Retinoid-related orphan receptor gamma (RORγ) is a transcription factor belonging to a sub-family of nuclear receptors that includes two closely related members RORα and RORβ. The nuclear hormone receptor RORγ regulates transcriptional genes involved in the production of the pro-inflammatory interleukin IL-17 which has been linked to autoimmune diseases such as rheumatoid arthritis, multiple sclerosis and inflammatory bowel disease. This transcriptional activity of RORγ is modulated through a protein-protein interaction involving the activation function 2 (AF2) helix on the ligand binding domain of RORγ and a conserved LXXLL helix motif on coactivator proteins. The conformation of the AF2 helix can be modulated through targeted ligands which bind the LBS and increase the binding of the coactivator protein (agonists) or disrupt binding (inverse agonists) thereby enhancing or inhibiting transcription.

However, extensive crystallization efforts with BIO399 and RORγ518 or other AF2 intact constructs did not produce crystals. We attributed the inability to form crystals to the unfolding of the AF2 helix induced by BIO399. We reasoned that if we could remove the unfolded AF2 helix using proteolysis we could produce a binary complex more amenable to crystallization. The Actinase E treated RORγ518 BIO399 ternary complex (aeRORγ493/4) co-crystallized readily in several PEG based conditions. The structure of aeRORγ493/4 BIO399 complex was solved to 2.3 Å and adopted a similar core fold to the BIO592 agonist crystal structure. BIO399 binds to the ligand binding site of RORγ adopting a collapsed conformation as seen with BIO592 where the two compounds superimpose with an RMSD of 0.72 Å. The majority of the side chains within 4 Å of BIO399 and BIO592 adopt similar rotomer conformations with the exceptions of Met358 and His479. The change in rotomer conformation of Met358 between the agonist and inverse agonist structures is attributed to the gem-dimethyl group on the larger 7 membered benzoxazinone ring system of BIO399. The comparison of the two structures shows that the agonist conformation observed in the BIO592 structure would be perturbed by BIO399 pushing Met358 into Phe506 of the AF2 helix indicating that Met358 is a trigger for inducing inverse agonism in RORγ. BIO399 neither orients the sidechain of Trp317 toward Tyr502 nor forms a hydrogen bond with His479 suggesting its mode of action is distinct from linear inverse agonists.

>[2x]GPTPEAPYTEIEHLVQSVCKSYRETCQLRLEDLLRQRSNIFSREEVTGYQRKSMWEMWERCAHHLTEAIQYVVEFAKRLSGFMELCQNDQIVLLKAGAMEVVLVRMCRAYNADNRTVFFEGKYGGMELFRALGCSELISSIFDFSHSLSALHFSEDEIALYTALVLINAHRPGLQEKRKVEQLQYNLELAFHHHLCKTHRQSILAKLPPKGKLRSLCSQHVERLQIFQ>[6x]AAAAANHSTQESGFDYEGLIDSELQKKRLDKSYRYFNNINRLAKEFPLAHRQREADKVTVWCSNDYLALS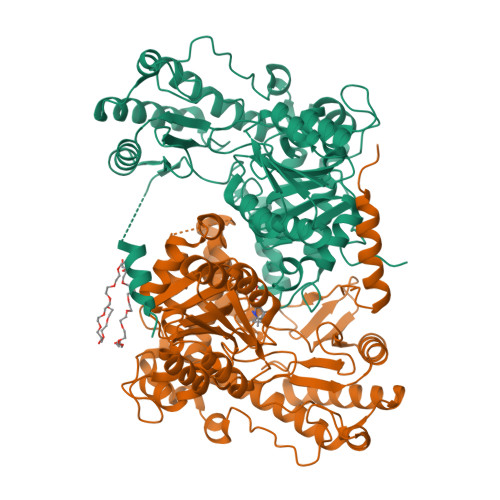KHPEVLDAMHKTIDKYGCGAGGTRNIAGHNIPTLNLEAELATLHKKEGALVFSSCYVANDAVLSLLGQKMKDLVIFSDELNHASMIVGIKHANVKKHIFKHNDLNELEQLLQSYPKSVPKLIAFESVYSMAGSVADIEKICDLADKYGALTFLDEVHAVGLYGPHGAGVAEHCDFESHRASGIATPKTNDKGGAKTVMDRVDMITGTLGKSFGSVGGYVAASRKLIDWFRSFAPGFIFTTTLPPSVMAGATAAIRYQRCHIDLRTSQQKHTMYVKKAFHELGIPVIPNPSHIVPVLIGNADLAKQASDILINKHQIYVQAINFPTVARGTERLRITPTPGHTNDLSDILINAVDDVFNELQLPRVRDWESQGGLLGVGESGFVEESNLWTSSQLSLTNDDLNPNVRDPIVKQLEVSSGIKQ pyrido[3,4-g]quinazolin-2-amine | C11 H8 N4 | 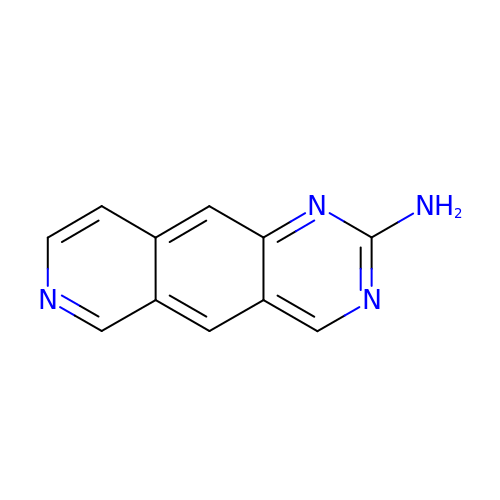HTMYPIWEXZOFDM-UHFFFAOYSA-N>GSRCPTECTCLDTVVRCSNKGLKVLPKGIPRDVTELYLDGNQFTLVPKELSNYKHLTLIDLSNNRISTLSNQSFSNMTQLLTLILSYNRLRCIPPRTFDGLKSLRLLSLHGNDISVVPEGAFNDLSALSHLAIGANPL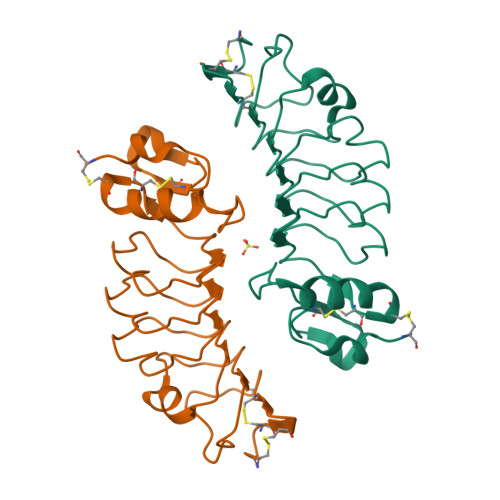YCDCNMQWLSDWVKSEYKEPGIARCAGPGEMADKLLLTTPSKKFTCAAAHHHHHH[2x]> MKEFYLTVEQIGDSIFERYIDSNGRERTREVEYKPSLFAHCPESQATKYFDIYGKPCTRKLFANMRDASQWIKRMEDIGLEALGMDDFKLAYLSDTYNYEIKYDHTKIRVANFDIEVTSPDGFPEPSQAKHPIDAITHYDSIDDRFYVFDLLNSPYGNVEEWSIEIAAKLQEQGGDEVPSEIIDKIIYMPFDNEKELLMEYLNFWQQKTPVILTGWNVESFDIPYVYNRIKNIFGESTAKRLSPHRKTRVKVIENMYGSREIITLFGISVLDYIDLYKKFSFTNQPSYSLDYISEFELNVGKLKYDGPISKLRESNHQRYISYNIIDVYRVLQIDAKRQFINLSLDMGYYAKIQIQSVFSPIKTWDAIIFNSLKEQNKVIPQGRSHPVQPYPGAFVKEPIPNRYKYVMSFDLTSLYPSIIRQVNISPETIAGTFKVAPLHDYINAVAERPSDVYSCSPNGMMYYKDRDGVVPTEITKVFNQRKEHKGYMLA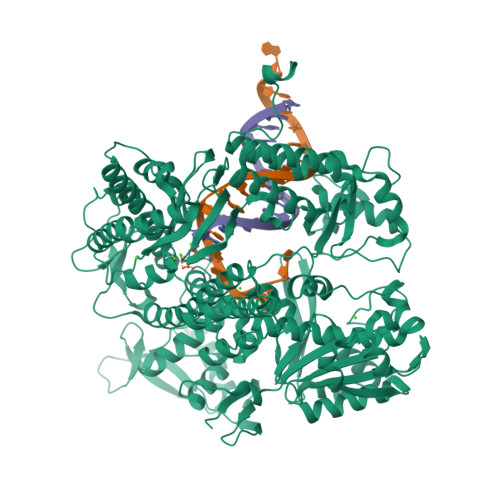AQRNGEIIKEALHNPNLSVDEPLDVDYRFDFSDEIKEKIKKLSAKSLNEMLFRAQRTEVAGMTAQINRKLLINSLYGALGNVWFRYYDLRNATAITTFGQMALQWIERKVNEYLNEVCGTEGEAFVLYGDTDSIYVSADKIIDKVGESKFRDTNHWVDFLDKFARERMEPAIDRGFREMCEYMNNKQHLMFMDREAIAGPPLGSKGIGGFWTGKKRYALNVWDMEGTRYAEPKLKIMGLETQKSSTPKAVQKALKECIRRMLQEGEESLQEYFKEFEKEFRQLNYISIASVSSANNIAKYDVGGFPGPKCPFHIRGILTYNRAIKGNIDAPQVVEGEKVYVLPLREGNPFGDKCIAWPSGTEITDLIKDDVLHWMDYTVLLEKTFIKPLEGFTSAAKLDYEKKASLFDMFDF> HHHHHHHSSGLVPRGSHMAIYADNSYSIGNTPLVRLKHFGHNGNVVVKIEGRNPSYSVKCRIGANMVWQAEKDGTLTKGKEIVDATSGNTGIALAYVAAARGYKITLTMPETMSLERKRLLCGLGVNLVLTEGAKGMKGAIAKAEEIVASDPSRYVMLKQFENPANPQIHRETTGPEIWKDTDGKVDVVVAGVGTGGSITGISRAIKLDFGKQITSVAVEPVESPVISQTLAGEE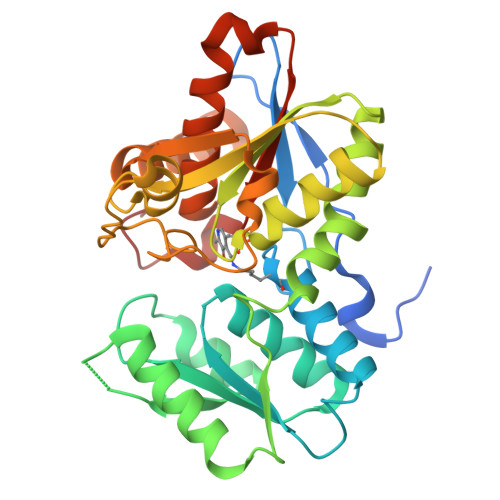VKPGPHKIQGIGAGFIPKNLDLSIIDRVETVDSDTALATARRLMAEEGILAGISSGAAVAAADRLAKLPEFADKLIVVILPSASERYLSTALFEGIEG>[4x]GSGDSGS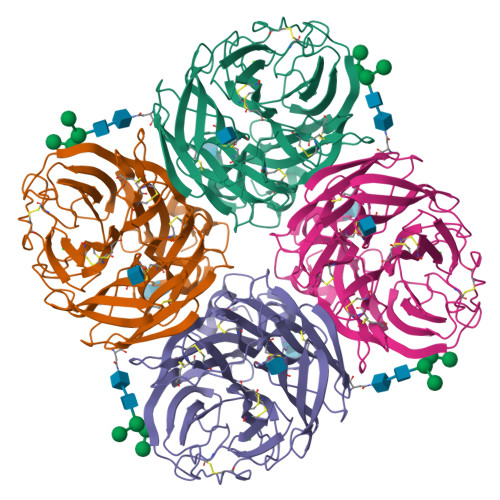PGLEYRNWSKPQCQITGFAPFSKDNSIRLSAGGDIWVTREPYVSCDHSKCYQFALGQGTTLNNKHSNSTIHDRTSHRTLLMNELGVPFHLGTKQVCIAWSSSSCHDGKAWLHVCVTGDDRNATASFVYNGMLVDSIGSWSRNILRTQESECVCINGTCTVVMTDGSASGRADTRILFIREGKIIHISPLSGSAQHIEECSCYPRYPNVRCVCRDNWKGSNRPVIDINMADYNINSSYVCSGLVGDTPRNDDSSSSSNCKDPNNERGNPGVKGWAFDNDNDVWMGRTISKDLRSGYETFKVIGGWTTANSKSQVNRQVIVDNNNWSGYSGIFSVEGKSCVNRCFYVELIRGGPQETRVWWTSNSIVVFCGTSGTYGTGSWPDGANINFMPI> SPSAEACGY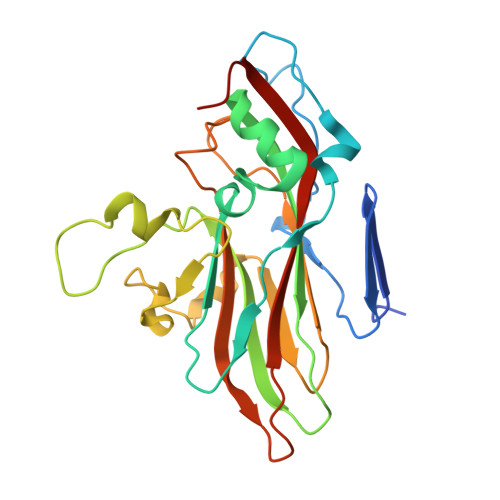SDRVLQLKLGNSAIVTQEAANYCCAYGEWPNYLPDHEAVAIDKPTQPETATDRFYTLKSVKWEAGSTGWWWKLPDALNNIGMFGQNVQHHYLYRSGFLIHVQCNATRFHQGALLVVAIPEHQRGAHNTNTSPGFDDIMKGEEGGTFNHPYVLDDGTSLACATIFPHQWINLRTNNSATIVLPWMNAAPMDFPLRHNQWTLAIIPVVPLGTRTMSSMVPITVSIAPMCCEFNGLRHAITQ> GSHMNGLIYAVGGYDGNTHLNSVEAYDPERNEWSLVAPLSTRRSGVGVAVLNGLIYAVGGYDGNTHLNSVEAYDPHHNEWSLVAPLSTRRSGVGVAVLNGLIYAVGGYDGNTHLNSVEAYDPERNEWSLVAPLSTRRSGVGVAVLNGLIYAVGGYDGNTHLNSVEAYDPH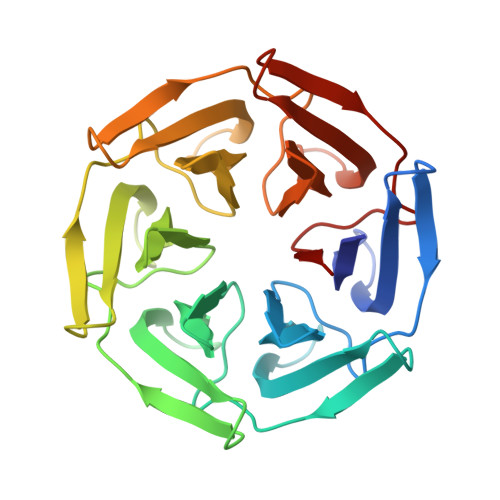HNEWSLVAPLSTRRSGVGVAVLNGLIYAVGGYDGNTHLNSVEAYDPERNEWSLVAPLSTRRSGVGVAVLNGLIYAVGGYDGNTHLNSVEAYDPHHNEWSLVAPLSTRRSGVGVAVL> MLGPKRCSMVLDVAFVLEGSDKIGEADFNRSKEFMEEVIQRMDVGQDSIHVTVLQYSYMVTVEYPFSEAQSKGDILQRVREIRYQGGNRTNTGLALRYLSDHSFLVSQGDREQAPNLVYMVTGNPASDEIKRLPGDIQVVPIGVGPNANVQELERIGWPNAPILIQDFETLP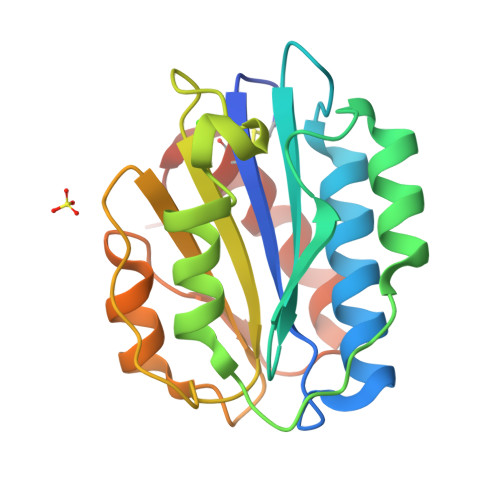REAPDLVLQRCSSGEGLEHHHHHH>MADLAESNIKVMC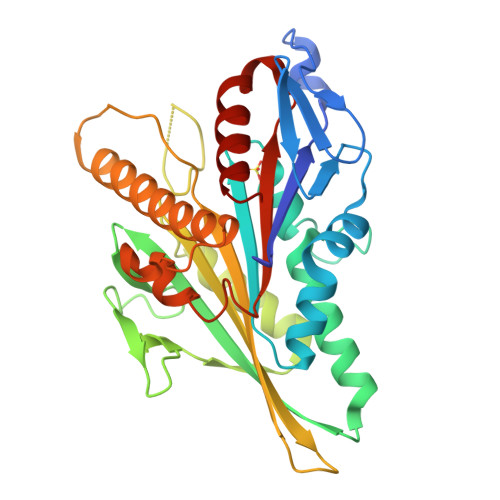RFRPLNESEVNRGDKYIAKFQGEDTVVIASKPYAFDRVFQSSTSQEQVYNDAAKKIVKDVLEGYNGTIFAYGQTSSGKTHTMEGKLHDPEGMGIIPRIVQDIFNYIYSMDENLEFHIKVSYFEIYLDKIRDLLDVSKTNLSVHEDKNRVPYVKGATERFVSSPDEVMDTIDEGKSNRHVAVTNMNEHSSRSHSIFLINVKQENTQTEQKLSGKLYLVDLAGSEKVSKTGAEGAVLDEAKNINKSLSALGNVISALAEGSTYVPYRDSKMTRILQDSLGGNARTTIVICCSPSSYNESETKSTLLFGQRAKTI[6x]> MGKGEGEVAGCKAAARLGVEGVFVEECFDGSYCRNLERIGYLRKGRLEPLEAAYQASRGMLCMGETRGWAAAVEVIAGLGLSLDTALVYFD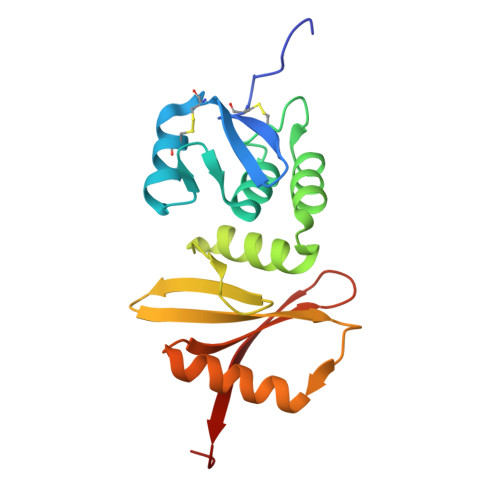LRRKGRKPLVGVRRGTLVYEHGGRVYEVLVLSEGYPLKIGSLVEWSRGASMDNHSPIVAIVDRTGLITYYEARAVRSIQ> ASVVIRNLSEATHNAIKFRARAAGRST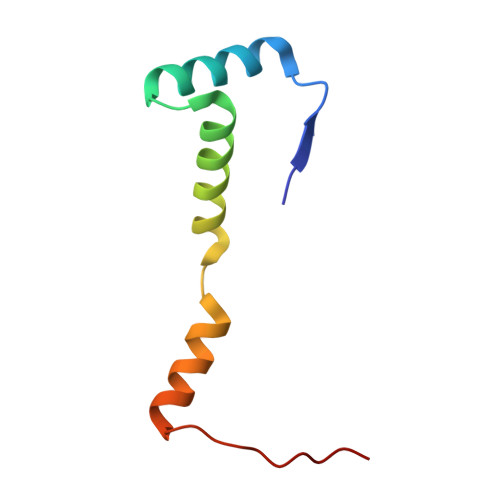EAEIRLILDNIAKAQQTVRLGSMLASIGQEIGGVELEDVRG>[4x]MDFGSLETVVANSAFIAARGSFDASSGPASRDRKYLARLKLPPLSKCEALRESLDLGFEGMCLEQPIGKRLFQQFLRTHEQHGPALQLWKDIEDYDTADDALRPQKAQALRAAYLEPQAQLFCSFLDAETVARARAGAGDGLFQPLLRAVLAHLGQAPFQEFLDSLYFLRFLQWKWLEAQPMGEDWFLDFRVLGRGGFGEVFACQMKATGKLYACKKLNKKRLKKRKGYQGAMVEKKILAKVHSRFIVSLAYAFETKTDLCLVMTIMNGGDIRYHIYNVDEDNPGFQEPRAIFYTAQIVSGLEHLHQRNIIYRDLKPENVLLDDDGNVRISDLGLAVELKAGQTKTKGYAGTPGFMAPELLLGEEYDFSVDYFALGVTLYEMIAARGPFRARGEKVENKELKQRVLE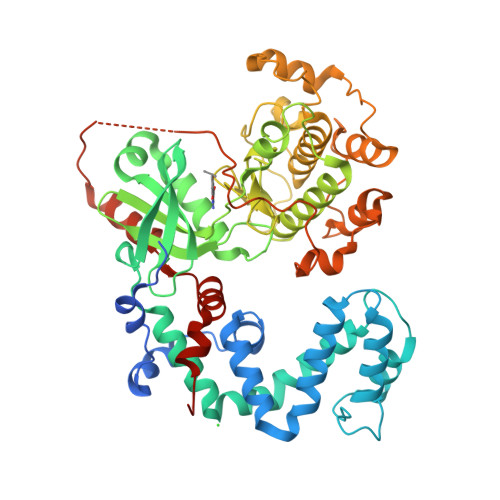QAVTYPDKFSPASKDFCEALLQKDPEKRLGFRDGSCDGLRTHPLFRDISWRQLEAGMLTPPFVPDSRTVYAKNIQDVGAFSTVKGVAFEKADTEFFQEFASGTCPIPWQEEMIETGVFGDLNVWRPDGHHHHHH Thiopeptides are a class of sulfur-rich, highly modified peptide antibiotics that are active against various drug-resistant bacterial pathogens. In contrast, the amino group of the terminal amide moiety in nosiheptide is endogenous and derives from an extended Ser residue of the precursor peptide34. Dehydration of this residue at the early stage in the nosiheptide biosynthetic pathway generates enamide, and subsequent dealkylation requires the activity of NosA, which has recently been characterized as a new terminal amide synthase, leading to a Cα-N bond cleavage for nosiheptide maturation with release of the co-product pyruvate. In conclusion, we characterized three key elements (basic lysine, acidic glutamic acid and flexible C-terminal loop) for the terminal amide formation in nosiheptide-represented thiopeptide biosynthesis, these mechanistic studies on how NosA works present an intriguing paradigm about how NosA family members function during thiopeptide biosynthesis.

We thus overexpressed NosA1-111 variant and its Se-Met form, and purified them to homogeneity for crystallization. The three-dimensional (3D) structure of NosA1-111 was determined using the single-wavelength anomalous-dispersion (SAD) method. Three monomers occupy one asymmetric unit, two of them form a dimer. Each monomer is identical to the others with an RMSD value of 0.21 Å for the backbone Cα atoms in the secondary structural regions, consisting of four anti-parallel β-sheets (β1, β2, β3, and β4), three α-helices (α1, α2 and α3) and six loops (L1, L2, L3, L4, L5 and L6), which are arranged in the order of β1- L1- α1- L2- β2- L3- β3- L4- α2- L5- α3- L6- β4. The first six or fewer residues at the N-terminus are invisible in all monomers, and the residues from 35 to 42 are also invisible in the two monomers that form a dimer conformation. This dimeric structure adopts a global fold, resembling an elliptic β-barrel of 28.9 Å in height, with diameters of 15 Å and 23 Å. The β-barrel is formed through several hydrogen bonds between the residues of the β4 strand in one monomer and the β2’ strand in another monomer, including hydrogen bonds between the E101 carboxyl and S53’ –OH group or R29’ imide group, between the S99 backbone carboxyl and the S53’ backbone nitrogen, and between the S99 backbone nitrogen and the S53’ carboxyl; and a hydrogen bond between the Y97 backbone oxygen and the S54’ side-chain –OH group. The β-barrel is also stabilized by salt bridge within the β-barrel between the side chains of the R96 and E94’ residues. However, the enzymatic assay performed on the HPLC system indicates that NosA1-111 has no catalytic activity, revealing that the C-terminal loop NosA112-151 is extremely important to the catalytic reaction.

>MTEHPAQQLYCTVVLWDLSRSAATVASLRAYLRDHAVDAYTTVPGLRQKTWISSTGPEGEQWGAVYLWDSPEAAYGRPPGVSKVVELIGYRPTERRYYSVEAATEGPAAAAAPFGKGLGLAFDPASPEPLTRPQEFVPPGADAFIPSRPPA[3x]>HHHHHHSSGLVPRGSHMASMSKVGINGFGRIGRLVLRRLLEVKSNIDVVAINDLTSPKILAYLLKHDSNYGPFPWSVDFTEDSLIVDGKSIAVYAEKEAKNIPWKAKGAEIIVECTGFYTSAEKSQAHLDAGAKKVLISAPAGEMKTIVYNVNDDTLDGNDTIVSVASATTNCLAPMAKALHDSFGIEVGTMTTIAAYTGTQSLVDGPRGKDLRASRAAAENIIPHTTGAAKAIGLVIPELSGKLKGHAQRVPVKTGSVTELVSILGKKVTAEEVNNALKQATTNNESFGYTDEEIVSSDIIGSHFGSVFDATQTEITAVGDLQLVKTVAWYDNEYGFVTQLIRTLEKFAKL[4x]

Glyceraldehyde-3-phosphate dehydrogenase (GAPDH) is a highly conserved enzyme involved in the ubiquitous process of glycolysis and presents a loop (residues 208–215 of Escherichia coli GAPDH) in two alternative conformations (I and II). In the presence of inorganic phosphate (Pi), GAPDH catalyzes the conversion of D-glyceraldehyde-3-phosphate (G3P) to 1,3-diphosphoglycerate (BPG), accompanying the reduction of NAD+ to NADH. All the structures reported in this paper have four subunits: O, P, Q, and R. Each subunit contained two domains: the C-terminal catalytic domain and the N-terminal NAD+-binding domain. Two anion recognition sites, “Ps” and “Pi”, bind the C3 phosphate of G3P and inorganic phosphate, respectively.

Two novel G3P-binding forms were observed in the ternary complexes WT.NAD.G3P and C150A+H177A.NAD.G3P. In these structures, the C3 phosphates of G3P are all located in the “Ps” site, while the “new Pi” site remains unoccupied. First, in the P subunit of C150A+H177A.NAD.G3P, the oxygen atom O1P of the C3 phosphate forms hydrogen bonds with the Oγ atoms of Thr182 and Thr180, as well as with NH1 of Arg232. However, it is the O3P oxygen atom that forms hydrogen bonds with the same amino acid in the Q subunit. The second difference is the orientation of O1 and O2 in G3P. In the P subunit, O1 of G3P forms hydrogen bonds with Nε of His207, and one water molecule, while O2 of G3P forms hydrogen bonds with water. However, in the Q subunit, the O1 of G3P forms hydrogen bonds with Oγ and the amide nitrogen of Thr151, while the O2 of G3P interacts with the amide nitrogen of Ala150. The G3P of the O subunit of C150A+H177A.NAD.G3P is present in hydrate form. We compared the G3P-binding form in the wild type and mutants, and found that after mutation, the catalytic cavity is increased almost 10 Å3 in C150A+H177A.This is helpful for G3P to move.>[4x]GITGTWYNQLGSTFIVTAGADGALTGTYESAVGNAESRYVLTGRYDSAPATDGSGTALGWTVAWKNNYRNAHSATTWSGQYVGGAEARINTQWLLTSGTTEANAWKSTLVGHDTFTKVK

In this work, we use SPA cryo-EM with VPP and Cs-corrector to determine the structure of SA with a molecular weight of ~52 kDa. Different from hemoglobin that consists mostly of α-helices, SA is constituted by mainly β-strands. Our work demonstrates that the VPP can be used in SPA to resolve SA in both the apo-state and biotin-bound state at near-atomic resolution. The atomic model of SA solved previously by X-ray crystallography (PDB 1MEP28) can fit into the EM densities with a correlation coefficient ~0.74, indicating the structural fidelity of SA in its crystallographic and soluble forms.

In the end, we obtained a reconstruction of apo-SA at 3.3 Å resolution (with D2 symmetry applied during the refinement) from a final dataset composed of ~24,000 particles and a reconstruction of the SA–biotin complex at 3.2 Å resolution (with D2 symmetry applied during the refinement) from a final dataset comprising ~45,000 particles. Compared with the biotin-bound SA, the density corresponding to loop 46–51 in the EM map of apo-SA was missing, indicating that this lid-like loop is flexible without ligand binding. We performed this 3D skip-alignment classification analysis of the apo-SA and biotin-SA datasets separately, and found a rather small occupancy variance around the biotin-binding pocket among the different classes in each dataset, demonstrating unambiguously the lack of biotin in all the monomers of apo-SA and the full occupancy of biotin in all the monomers of biotin-SA. We noticed that even after the careful scrutiny of the SA particle images by 2D classification to remove all obvious junk or bad particles, only ~20% (79, 289 vs. 378, 987 for the apo-SA) of the seemingly good particles contributed to the correct high-resolution reconstruction after the 3D classification. Based on the location of each particle, the 212,105 particles were manually divided into two subsets with 134,606 particles in the clustering regions (subset A) and 77,499 particles in the uniformly dispersed regions (subset B). We immediately noticed that among the 44,326 particles, 35,676, accounting for >80%, were from subset A and only 8,650, accounting for <20%, were from subset B. The fact that the contribution of the particles from subset A to the best 3D class increased from 63.5% (134,606/212,105) to 80.5% (35,676/44,326) after the classification indicates that a larger portion of the molecules on the GWI were well-preserved. The maps from subset A consistently demonstrated the correct features of the SA molecule, whereas the maps from subset B were of poor quality. To further investigate the effect of AWI on the structure of SA molecules, we performed cryo-EM analysis of apo-SA on regular holey carbon grids without graphene support. SPA of these SA molecules demonstrated a strong preferential orientation, which is similar to that of subset B in the above analysis.>[3x]GPGSATTVHGETVVNGAK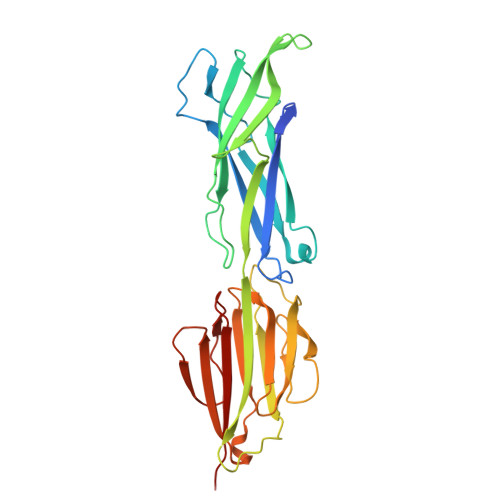LTVTKNLDLVNSNALIPNTDFTFKIEPDTTVNEDGNKFKGVALNTPMTKVTYTNSDKGGSNTKTAEFDFSEVTFEKPGVYYYKVTEEKIDKVPGVSYDTTSYTVQVHVLWNEEQQKPVATYIVGYKEGSKVPIQFKASLDSTTLTVKKKVSGTGGDRSKDFNFGLTLKANQYYKASEKVMIEKTTKGGQAPVQTEASIDQLYHFTLKDGESIKVTNLPVGVDYVVTEDDYKSEKYTTNVEVSPQDGAVKNIAGNSTEQETSTDKDMTITFTNKKVFE> KENGKRTEVKIGAK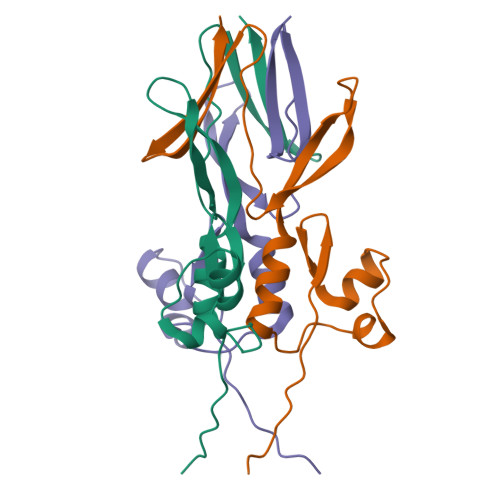TSVMKEKDGKLFTGKANKETNKVDGANATEDADEGKGLVTAKDVIDAVNKTGWRIKTTDANGQNGDFATVASGTNVTFASGNGTTATVTNGTDGITVKYDAK> MLKRKQSSRVEAQPVTDFGPDESLSDNADILWINKPWVHSLLRICAIISVISVCMNTPMTFEHYPPLQYVTFTLDTLLMFLYTAEMIAKMHIRGIVKGDSSYVKDRWCVFDGFMVFCLWVSLVLQVFEIADIVDQMSPWGMLRIPRPLIMIRAFRIYFRFELPRTRITNILKRSGEQIWSVSIFLLFFLLLYGILGVQMFGTFTYHCVVNDTKPGNVTWNSLAIPDTHCSPELEEGYQCPPGFKCMDLEDLGLSRQELGYSGFNEIGTSIFTVYEASSQEGWVFLMYRAIDSFPRWRSYFYFITLIFFLAWLVKNVFIAVIIETFAEIRVQFQQMWGTRSSTTSTATTQMFHEDAAGGWQLVAVDVNKPQGRAPACLQKMMRSSVFHMFILSMVTVDVIVAASNYYKGENFRRQYDEFYLAEVAFTVLFDLEALLKIWCLGFTGYISSSLHKFELLLVIGTTLHVYPDLYHSQFTYFQVLRVVRLIKISPALEDFVYKIFGPGKKLGSLVVFTASLLIVMSAISLQMFCFVEELDRFTTFPRAFMSMFQILTQEGWVDVMDQTLNAVGHMWAPLVAIYFILYHLFATLILLSLFVAVILDNLELDEDLKKLKQLKQSEANADTKEKLPLRLRIFEKFPNRPQMVKISKLPSDFTVPKIRESFMKQFIDRQQQDTCCLFRILPSTSSSSCDNPKRPTVEDNKYIDQKLRKSVFSIRARNLLEKETAVTKILRACTRQRMLSGSFEGQPAKERSILSVQHHIRQERRSLRHGSNSQRISRGKSLETLTQDHSNTVRYRNAQREDSEIKMIQEKKEQAEMKRKVQEEELRENHPYFDKPLFIVGREHRFRNFCRVVVRARFNASKTDPVTGAVKNTKYHQLYDLLGLVTYLDWVMITVTICSCISMMFESPFRRVMHAPTLQIAEYVFVIFMSIELNLKIMADGLFFTPTAVIRDFGGVMDIFIYLVSLIFLCWMPQNVPAESGAQLLMVLRCLRPLRIFKLVPQMRKVVRELFSGFKEIFLVSILLLTLMLVFASFGVQLFAGKLAKCNDPNIIRREDCNGIFRINVSVSKNLNLKLRPGEKKPGFWVPRVWANPRNFNFDNVGNAMLALFEVLSLKGWVEVRDVIIHRVGPIHGIYIHVFVFLGCMIGLTLFVGVVIANFNENKGTALLTVDQRRWEDLKSRLKIAQPLHLPPRPDNDGFRAKMYDITQHPFFKRTIALLVLAQSVLLSVKWDVEDPVTVPLATMSVVFTFIFVLEVTMKIIAMSPAGFWQSRRNRYDLLVTSLGVVWVVLHFALLNAYTYMMGACVIVFRFFSICGKHVTLKMLLLTVVVSMYKSFFIIVGMFLLLLCYAFAGVVLFGTVKYGENINRHANFSSAGKAITVLFRIVTGEDWNKIMHDCMVQPPFCTPDEFTYWATDCGNYAGALMYFCSFYVIIAY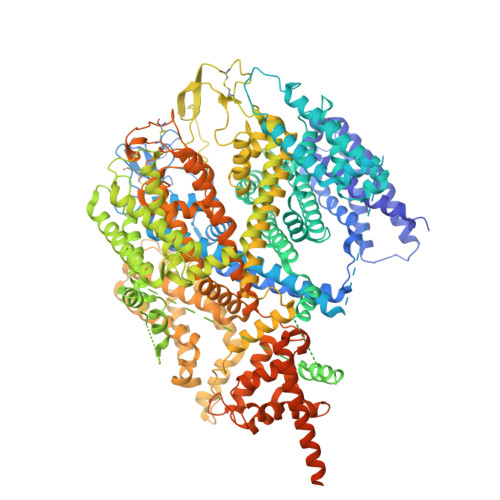IMLNLLVAIIVENFSLFYSTEEDQLLSYNDLRHFQIIWNMVDDKREGVIPTFRVKFLLRLLRGRLEVDLDKDKLLFKHMCYEMERLHNGGDVTFHDVLSMLSYRSVDIRKSLQLEELLAREQLEYTIEEEVAKQTIRMWLKKCLKRIRAKQQQSCSIIHSLRESQQQELSRFLNPPSIETTQPSEDTNANSQDHNTQPESSSQQQLLSPTLSDRGGSRQDAADTGKPQRKIGQWRLPSAPKPISHSVSSVNLRFGGRTTMKSVVCKMNPMPDTASCGSEVKKWWTRQLTVESDESGDDLLDI>[6x]MGESKRTEKTRVLVVGATGYIGKRIVRACLAEGHETYVLQRPEIGLEIEKVQLFLSFKKLGARIVEGSFSDHQSLVSAVKLVDVVVSAMSGVHFRSHNILVQLKLVEAIKEAGNVKRFLPSEFGMDPPRMGHALPPGRETFDQKMEVRQAIEAAGIPYTYVVGACFAAYFAGNLSQMVTLLPPKEKVNIYGDGNVKVVFADEDDIAKYTAKTLNDPRTLNKTVNIRPPDNVLTQLELVQIWEKLTGKELEKTNIAAQDFLANIEQMEIPHQAGIGHFYHIFYEGCLTDHEVGEDEEASSLYPDVKYKRMDDYLRMFL

Pinoresinol/lariciresinol reductase (PLR), an NADPH-dependent reductase, converts pinoresinol to lariciresinol and subsequently to secoisolariciresinol. Here, we present crystal structures of IiPLR1 from Isatis indigotica and pinoresinol reductases (PrRs) AtPrR1 and AtPrR2 from Arabidopsis thaliana, in the apo, substrate-bound and product-bound states. The crystal structures were captured in the apo, substrate-bound and/or product-bound forms. We found that, for all 16 structures we solved, each enzyme adopts a similar head-to-tail dimer conformation, strongly suggesting that each PLR/PrR functions as a homodimer, consistent with the literature that TpPLR1 exists as a dimeric entity in solution. Each structure contains a head-to-tail homodimer, and the catalytic pocket comprises structural elements from both monomers. β4 loop covers the top of the pocket, and residue 98 from the loop governs catalytic specificity.

In contrast to IiPLR1_NAP_ + PIN, the β4 loops of AtPrR1_NAP_ + PIN and AtPrR2_NAP_ + PIN can be clearly identified. These well-defined loops twist as an “8” shape and cover both the NADP+-binding and substrate-binding grooves. Within the twisted loop, His93 and His97 “grasp” helices α5 and α10, while Val92 and Phe94 interact directly with (+)-pinoresinol; Arg95 strongly interacts with NADP+ as well as each of the GXXGXXG motif and α2-helix from neighboring protomer of the dimer. Similar β4 loops are also observed in all other AtPrR1 substrate/product-bound structures, whereas each β4 loop is disordered in the corresponding IiPLR1 structures, which indicates that the β4 loop may participate in substrate selectivity and, hence, catalysis. Furthermore, Leu46 (corresponding to Val46 in IiPLR1), His276 and Phe277 of AtPrR1 are positioned similar to the corresponding residues of IiPLR1 to effect substrate binding or product release, except that the β4 loops cover the substrate/product, which are disordered in the IiPLR1 structures. Importantly, the PrRs have more strict requirements for the binding and orientation of lariciresinol compared with PLRs, so PrRs cannot efficiently carry out the third step.>MASRGVNKVILVGNLGQDPEVRYMPSGGAVANFTLATSESWRDKQTGEMKEQTEWHRVVLFGKLAEVAGEYLRKGSQVYIEGQLRTRKWTDQSGQDKYTTEVVVNVGGTMQMLGGRQGGGAPAGGGQQQGGWGQPQQPQGGNQFSGGAQSRPQQQAPAAPSNEPPMDFDDDIPFHHHH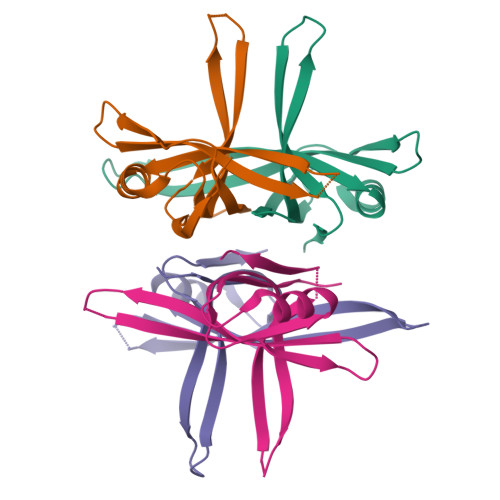HH[4x]>[2x]QVASEYLGGPGGDAFDDKALAQNGDITRIEMQCTDVATYIKLRYGKVDSRQWGWANENCIQ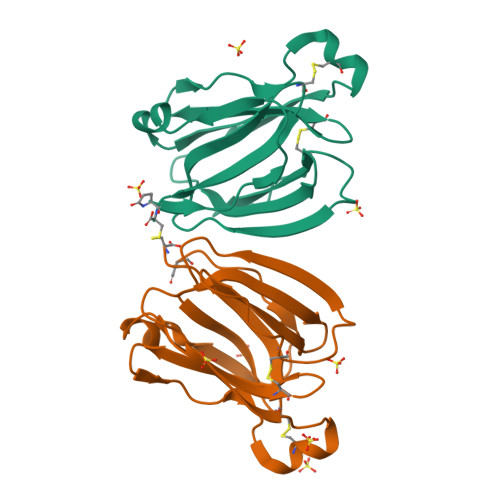WSKKGVKVVHELSSGEYITSAIVTYGKYVQSITFKTNKRTLPRCGTSATEKSVTVLIPGGLKYISGRWGCRIDGLRFHAKC[1-(2-hydroxyethyl)pyrazol-4-yl]methyl (2S)-1-[(2S)-2-cyclohexyl-2-(3,4,5-trimethoxyphenyl)ethanoyl]piperidine-2-carboxylate | C29 H41 N3 O7 | 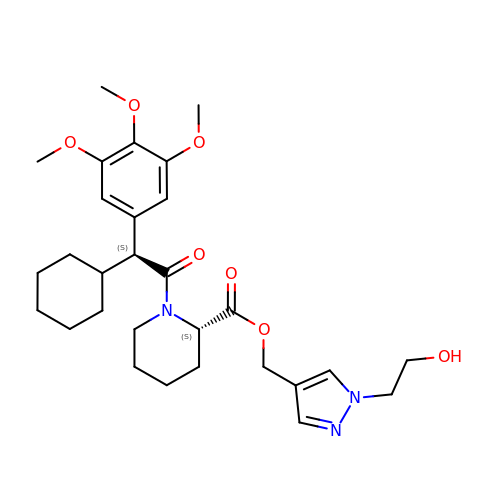NKOOEKXFGPRCRA-OZXSUGGESA-N> MNGYDPVLLSRILTELTLTVHIIYATIGVGVPLMIAIAQWVGIRKNDMHYILLARRWTRGFVITVAVGVVTGTAIGLQLSLLWPNFMQLAGQVISLPLFMETFAFFFEAIFLGIYLYTWDRFENQKKHLLLLIPVAIGSSASAMFITMVNAFMNTPQGFELKNGELVNIDPIVAMFNPAMPTKVAHVLATSYMTSAFVLASIAAWHLWKGNRHIYHRKALHLTMKTAFIFSVASALVGDLSGKFLAEYQPEKLAAAEWHFETSSHAPLILFGTLEEDNEVKYALEIPYALSILAHNHPAAVVTGLNDIPEDERPPLYIHYLFDVMVTIGVFLMVVAAVYW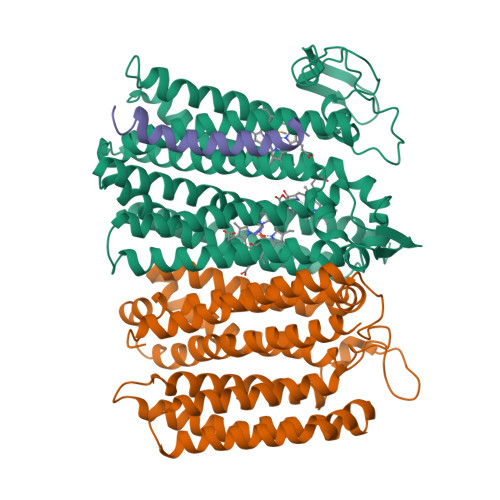LGSIFRWKWTAKNWFFGLLVAGGPLAMIAIEAGWYLAEVGRQPWILRGYMKTAEGATTSAHVDTMLVLFCLLYIVLVIASATVLIRMFRRNPVERELEERANRGEVAP;> MTLEVIGISVLWLFLFGYIIVASIDFGAGFFSVYSHWANQQHILHRIIQRYLSPVWEVTNVFLVFFFVGIVGFFPKTAYYYGSILLVPASIAIVLLAIRGSYYAFHTYGETERNWYLLAYGLTGLFIPASLSIVLTISEGGFVEENAAGVALDYGKLFASPLSWSVVLLSVTSVLYISAVFLTYYADAAGDEQARALLRRYALLWSGPTMLSALLIIYQLRYHNPEHYDNLWNVAWMLVISFLFFVITVWLLGRQRRFGWAFIALLFQYAFAFYAYGISHYPYLLYPYLTIYDGFTNETMAMALIVAFIAGLLLLIPSLYLLMRLFLFNKAYVKGKWEGGKG;> MQTFLIMYAPMVVVALSVVAAFWVGLKDVHVNE>[2x]GPGSEVPADGNAGLLAEPQIAMFCGKLNMHMNVQNGKWESDPSGTKTCIDTKEGILQYCQEVYPELQITNVVEANQPVTIQNWCKRGWKQCNGHPHIVVPYRCLVGEFVSDALLVPDKCKLLHQERMDVCETHLHWHTVAKESCSEKSMNLHDYGMLLPCGIDKFRGVEFVCCPLAEESDNLDS;>GSTGSPPGPPEDVTIDEITDTTAQLSWRPGADNHSPITMYVVQARTPFSVGWQAVSTVPEVIDGKTFTATVVGLNPWVEYEFRVVAANLIGIGEPSRPSENRRTEEALPEVTPANVSGGGGSKSELVITWETVPEELQNGGGFGYVVAFRPFGTISWMQTVVASPDASRYVFRNESLPPFSPYEVKVGVYNNKGEGSFSPVTVVYSAEEEPTRAPITVLARSLSATDIEISWAPPRENQHKGRIQGYEVRCWRHDEKEENARKIRTVGNQTSAKVTNLQGNALYHLAVKAYNTAGTGPSSAMVNVTTKK[2x]

Contactins (CNTNs) are neural cell adhesion molecules that encode axon-target specificity during the patterning of the vertebrate visual and olfactory systems. Because CNTNs are tethered to the plasma membrane by a glycosylphosphatidylinositol anchor, they lack an intracellular region to communicate across the membrane. Instead, they form coreceptor complexes with distinct transmembrane proteins to transmit signals inside the cell. Finally, structural analyses of five CNTN–amyloid pairs indicate that these proteins interact through a conserved interface involving the second fibronectin type III repeat of CNTNs and the copper-binding domain of amyloid proteins.

We first sought to gain structural insights into CNTN–amyloid interactions by focusing on the CNTN4–APP complex. Because human APP(E1) seemed prone to aggregation, we attempted crystallization of the chicken and mouse complexes. Although both the chicken and mouse complexes crystallized, only the former yielded crystals that diffracted well enough to allow structure determination. Overall, there is little change in the E1 domain of chicken APP compared with the published E1 domain of mouse APP ((36), RMSD of 0.475 Å over 155 Cα residues), which is not surprising given the 94% amino acid identity between the two proteins. The FN1–FN3 region of chicken CNTN4 is characterized by a sharp bend between the FN2 and FN3 domains that appears to be a hallmark of vertebrate CNTNs. The binding site involves the second FN repeat of CNTN4 and the copper-binding domain of APP, though it does not overlap with residues involved in copper binding. The complex interface occludes only ∼600 Å2 of surface area, but with a high shape complementarity coefficient of 0.78, which is consistent with values calculated for trypsin–trypsin-inhibitor structures. The interface is stabilized by a network of main chain–main chain hydrogen bonds between two antiparallel β-strands found in APP (L127–P130) and in CNTN4 (W748–Q750), respectively. In addition, the side-chain oxygen atom of S124 in APP forms a hydrogen bond with T751 in CNTN4, whereas its main chain oxygen atom forms a hydrogen bond with the side chain of Y761. In the chicken CNTN4–APP complex, A126 forms van der Waals interactions with the side-chain atoms of M749, Y761, and F763.> MTTLSGKTAIVGVAESDQIGKVPDKPAIALHAEAALNALEEAGLTLRDVDGLLTAGISPLELGEYLGIEPSYTDGTAVGGSSFVIHLAHAAAAIVTGRCSVALITHGESGRSRVGMPPRVPAPDSLRGQFEDPYGLPTPVGAYALACSRHMAEYGTTKEQLAEIAVATRKWAMLNPKAYMRDPITIEDVLNSRPIVWPFNLLDCCLVTDAGGACVVTSIERARDLRQHPVAILGVGESHDHSIISQMPSLTSFAARRSGQAAFKMAGVTHDDIDLAMIYDSFTYTVLLSLEDLGFCAKGEGGAFVSGQRTAPGGDFPMNTNGGGLSYTHPGMYGMFAIIEAVRQLRHDYADQGIRQ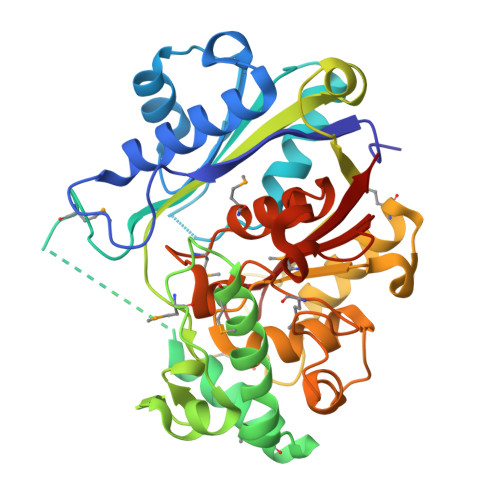VPNCELAIVHGTGGVLSSAGTAILGRV> GMENKVLYAYVQKD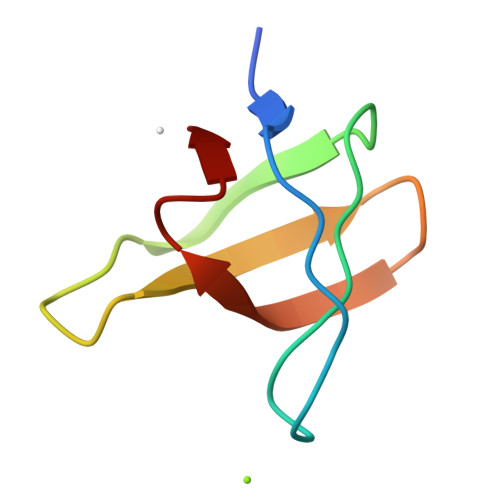DDEITITPGDKISLVARDTGSGWTKINNDTTGETGLVPTTYIRI>[4x]SNAMVYPVKHSPLLRQPEHFIARDELKALIQKVTHNLVNIKDETGEFLLRLDDGRVIDTKGWAGWEWTHGVGLYGMYHYYQQ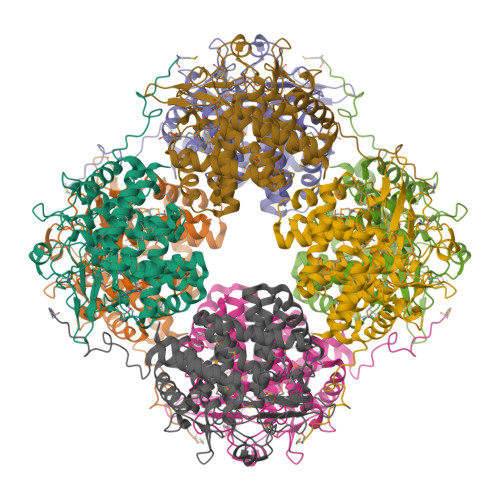TGDQTMRKIIDDWFADRFAEGATTKNVNTMAPFLTLAYRYEETRNPAYLPWLETWAEWAMNEMPRTDHGGMQHITLAEENHQQMWDDTLMMTVLPLAKIGKLLNRPEYVEEATYQFLLHVQNLMDKETGLWFHGWSYDGHHNFANARWARGNSWLTIVIPDFLELLDLPENNAVRRYLVQVLNAQIAALAKCQDESGLWHTLLDDPHSYLEASATAGFAYGILKAVRKRYVERHYAQVAEKAIRGIVKHISPEGELLQTSFGTGMGHDLDFYRHIPLTSMPYGQAMAMLCLTEYLRNYF N-{4-[(3-aminopropyl)amino]butyl}acetamide | C9 H21 N3 O | 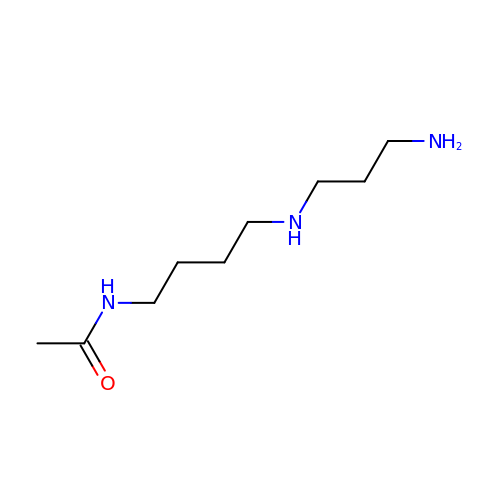FONIWJIDLJEJTL-UHFFFAOYSA-N4-[2-AMINO-5-(3,4,5-TRIMETHOXYPHENYL)PYRIDIN-3-YL]BENZOIC 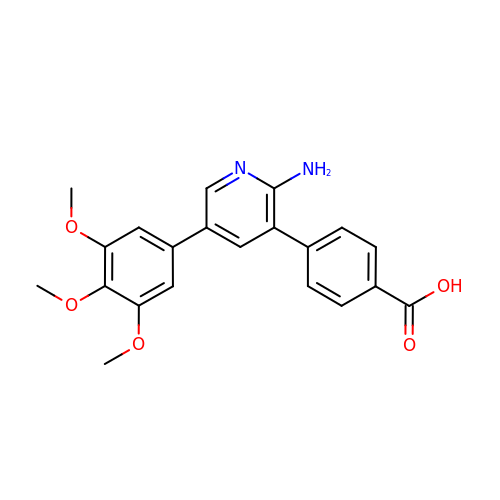ACID | C21 H20 N2 O5 | MWVUNZGIJWXHFJ-UHFFFAOYSA-N> MLRINSDAPNFDADTTVGKINFYDYLGDSWGVLFSHPADFTPVCTTEVSAFAKLKPEFDKRNVKLIGLSVEDVESHEKWIQDIKEIAKVKNVGFPIIGDTFRNVAFLYDMVDAEGFKNINDGSLKTVRSVFVIDPKKKIRLIFTYPSTVGRNTS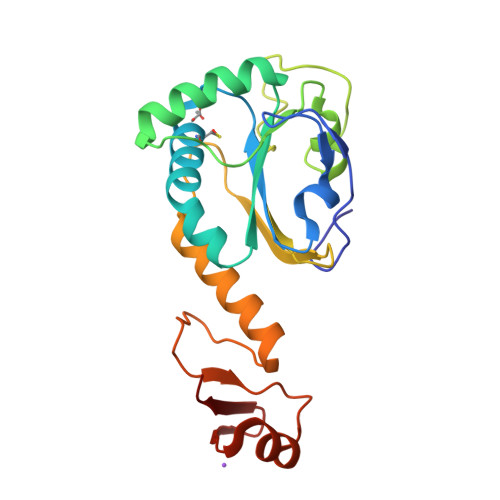EVLRVIDALQLTDKEGVVTPINWQPADDVIIPPSVSNDEAKAKFGQFNEIKPYLRFTKSK> ETPPRFTRTPVDQTGVSGGVASFICQATGDPRPKIVWNKKGKKVSNQRFEVIEFDDGSGSVLRIQPLRTPRDEAIYECVASNNVGEISVSTRLTVLREDQIPRGFPTIDMGPQLKVVERTRTATMLCAASGNPDPEITWFKDFLPVDTSNNNGRIKQLRSESIGGTPIRGALQIEQSEESDQGKYECVATNSAGTRYSAPANLYVRELREVRRVPPRFSIPPTNHEIMPGGSVNITCVAVGSPMPYVKWMLGAEDLTPEDDMPIGRNVLELNDVRQSANYTCVAMSTLGVIEAIAQIT;> SADGCTDWSIDIKKYQVLVGEPVRIKCALFYGYIRTNYSLAQSAGLSLMWYKSSGPGDFEEPIAFDGSRMSKEEDSIWFRPTLLQDSGLYACVIRNSTYCMKVSISLTVGENDTGLCYNSKMKYFEKAELSKSKEISCRDIEDFLLPTREPEILWYKECRTKTWRPSIVFKRDTLLIRE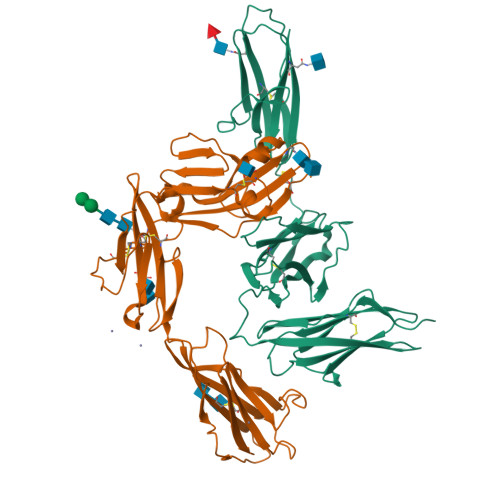VREDDIGNYTCELKYGGFVVRRTTELTVTAPLTDKPPKLLYPMESKLTIQETQLGDSANLTCRAFFGYSGDVSPLIYWMKGEKFIEDLDENRVWESDIRILKEHLGEQEVSISLIVDSVEEGDLGNYSCYVENGNGRRHASVLL N-[4-({[5-(DIMETHYLAMINO)-1-NAPHTHYL]SULFONYL}AMINO)BUTYL]-3-SULFANYLPROPANAMIDE 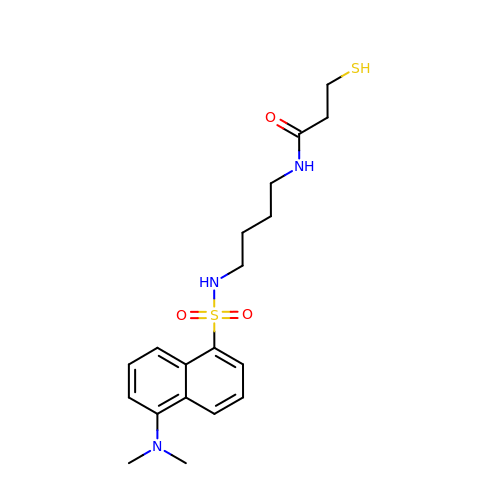| C19 H27 N3 O3 S2 | XPCVYJATJSZGJU-UHFFFAOYSA-N> KAFRRPVGIVHVKVVRAVGLRKKDLMGGADPFVKIKLSEDKIPSKKTTVKHKNLNPEWNEEFKFSVRDPQTQVLEFSVYDWEQVGNPEKMGMNVLALKEMVPDEHKAFTLELRKTLDGGEDGQPPDKYRGKLEVE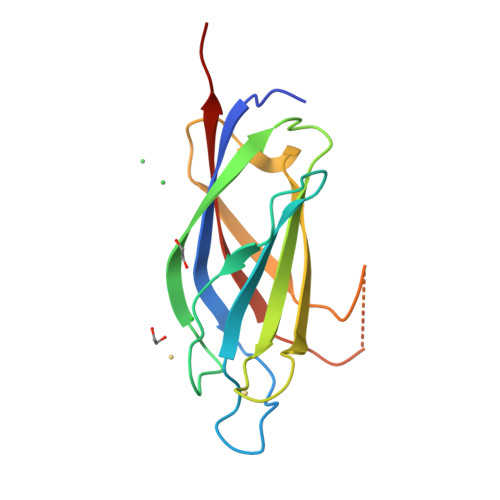LLYKPFTEEE> GPLGSPEFMSGSTLLKETGPREVFCGLTSIVWLHRRMPDAFFLVVGSRTCAHLIQSAAGVMIFAEPRFGTAILEERDLAGLADAHEELDRVVKSLLKRRPEIRTLFLVGSCPSEVIKIDLSRAAERLSSQFNGQVRILNYSGSGIETTFTQGEDGALKALVPLMPSSQEEQLLLAGTLANPVEDRLKTIFNRLGIQKVESFPPRESTKLPAIGPGTKVLLAQPYLTDTARELKDRGAEILQAPFPLGVEGSQ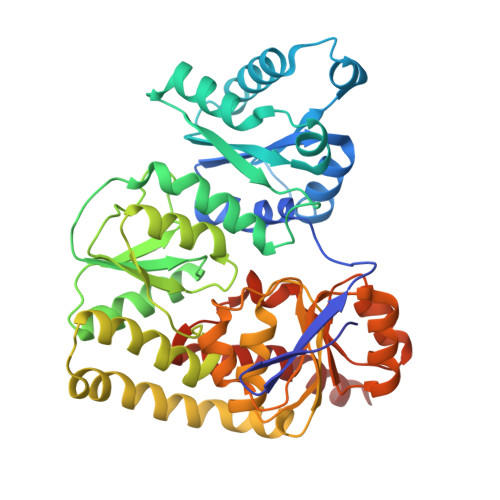LWIEAAANAFKIKKTLVDATLEPLITRAHKALKPYVEQLSGKKLFLLPESQLEIPLARFLSNECGMKLIEVGVPYLNREMMGPELDLLPQNTRIVEGQHVEKQLDRVREHHPDLVVCGMGLANPLEAEGISTKWSIEMVFSPIHGIDQASDLAELFARPLHRQNLLNKKTLEAV> GPLGSADDDLAAADKYADERKKVMCEDALCSNLSVENAAEILILADLHSADQLKTQAVDFINYHASDVLETSGWKSMVVSHPHLVAEAY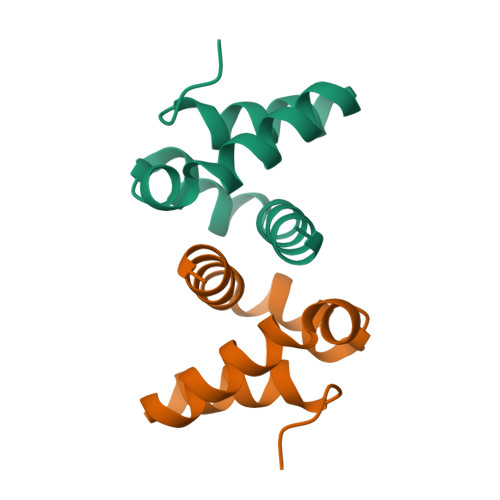RSLASAQCPFLGPPRKRLKQS> GSHMDADGKLLTEGGENENLRKNASKKETSLFQGFKSYLPIAELAI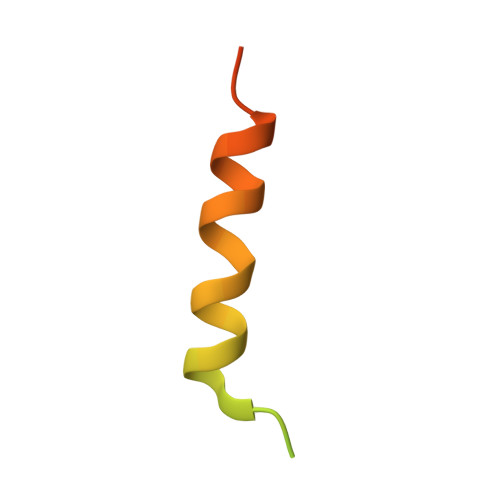ENTERLNY> MEYENALGIFSPDGRLIQVEYAQQASEQGSLVVFSSDTNEICLSIETKTHNKMLIDQNKLLPVDKDLNIWYTFSGIKPDSYKVLNEARLICRNYKIKTGTNISFDELAYELSLYKQKFTLDSSMRPFGIRSILLQVKDMAKIYVLEPDGNYSEYKCG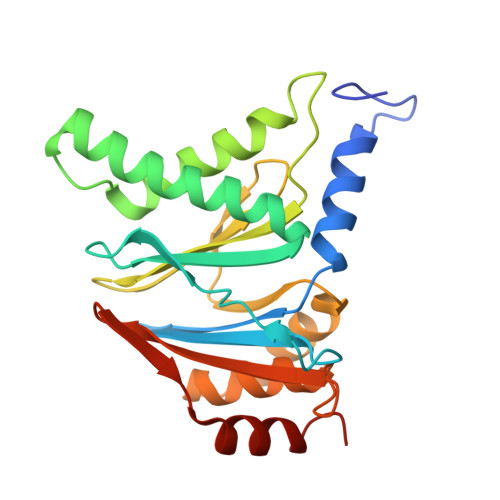AVGQKSVSVCEYLEKCEEEDIIFRSVSGLGTVVQSDKNKVMSYVISKDEIRRVEDETVSQIISTVSVK> HPETLVKVKDAEDQLGARVGYIELDLNSGKILESFRPEERFPLTSTFKVLLCGAVLSRVDAGQEQLGRRIHYSQNDLVEYSPVTEKHLTDGMTVRELCSAAITMSDNTAANLLLTTIGGPKELTDFLRQIGDKETRLDRIEPDLNEGKLGDLRDTTTPKAIASTLRKLLTGELLTLASRQQLIDWMEADKVAGPLLRSALPAGWFIADKSGAGERGSRGIIAALGPDGKPSRIVVIYTTGSQATMDERNRQIAEIGASLIKHW

The system of five interrelated, functional β-lactamases stems from the recombination of two homologs, the TEM-1 penicillinase and the PSE-4 carbenicillinase. We further expand this investigation to engineered enzyme variants by examining the same range of motions in a closely interrelated system composed of three recombined and functionally selected variants of TEM-1 and PSE-4, or ‘chimeras’. We thus demonstrate that a variety of non-native slow motions, including active-site motions that occur near the frequency of turnover, are compatible with β-lactamase activity in engineered variants.

The Ω-loop active-site wall contains the conserved Glu166, proposed to serve as a general base in the catalytic acylation and deacylation steps. Chimera cTEM-19m includes both segments of PSE-4 present in  either of the other chimeras, resulting in 19 substitutions on two active-site walls (S70 and Ω-loop walls) relative to TEM-1. Chimera cTEM-19m was most similar to cTEM-17m; both include segment 150–190 of PSE-4. Their active-site cavity volume (cTEM-19m: 741 Å3; cTEM-17m: 746 Å3) is nearly twice larger than the cavity of native TEM-1 (384 Å3), PSE-4 (427 Å3) and cTEM-2m (393 Å3). In cTEM-17m and cTEM-19m it is resolved in the m-30° conformation that swings the Tyr-phenoxy ring out of the active-site void, packing it against the cavity wall. This opens and increases the active-site volume relative to the t80° conformation observed in all other native and mutant apoenzyme structures of TEM-1 and PSE-4. The active-site volume is further increased in cTEM-17m and cTEM-19m by adoption of an open conformation of the active-site wall 214–218. The inclusion of 17 substitutions left cTEM-17m essentially unaltered relative to TEM-1, but inclusion of the substitutions Met68Leu/Met69Thr in cTEM-2m and cTEM-19m dropped kcat 1 to 3 orders of magnitude, to levels similar to PSE-4. The Y105 wall displayed slow dynamics in the three chimeras, with a 4-fold difference in kex for cTEM-17m (300 ± 90 s−1) and cTEM-19m (1,220 ± 230 s−1).> MTLI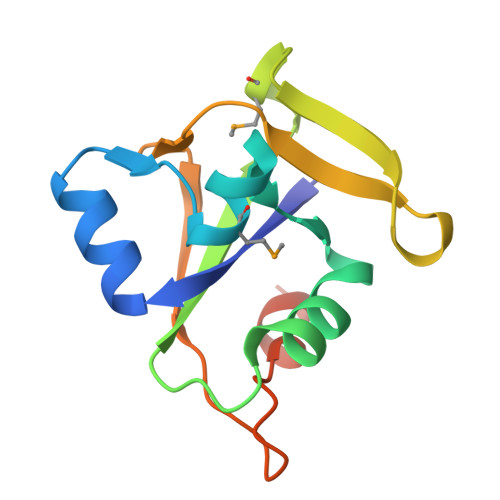YKILSRAEWDAAKAQGRFEGSAMDLADGFIHLSAGEQAQETAAKWFRGQANLVLLAVEAEPMGEDLKWEASRGGARFPHLYRPLLVSEVTREADLDLDADGVPQLGDHLALEHHHHHH>[2x]SNADRFAVSAEAENKVREQQPHVERIFSVGVSVLPKDCPDNPHIWLQLEGPKENASRAKEYLKGLCSPELQDEIHYPPKLHCIFLGAQGFFLDCLAWSTSAHLVPRAPGSLMISG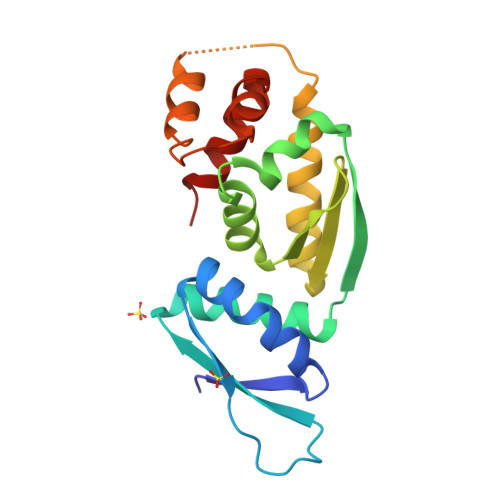LTEAFVMAQSRVEELAERLSWDFTPGPSSGASQCTGVLRDFSALLQSPGDAHREALLQLPLAVQEELLSLVQEA>AEIPLKYGATNEGKRQDPAMQKFRDNRLGAFIHWGLYAIPGGEWNGKVYGGAAEWLKSWAKVPADEWLKLMDQWNPTKFDAKKWAKMAKEMGTKYVKITTKHHEGFCLWPSKYTKYTVANTPYKRDILGELVKAYNDEGIDVHFYFSVMDWSNPDYRYDIKSKEDSIAFSRFLEFTDNQLKELATRYPTVKDFWFDGTWDASVKKNGWWTAHAEQMLKELVPGVAINSRLRADDKGKRHFDSNGRLMGDYESGYERRLPDPVKDLKVTQWDWEACMTIPENQWGYHKDWSLSYVKTPIEVIDRIVHAVSMGGNMVVNFGPQADGDFRPEEKAMATAIGKWMNRYGKAVYACDYAGFEKQDWGYYTRGKNDEVYMVVFNQPYSERLIVKTPKGITVEKATLLTTGEDITVVETTRNEYNVSVPKKNPGEPYVIQLKVRAAKGTKSIYR[4x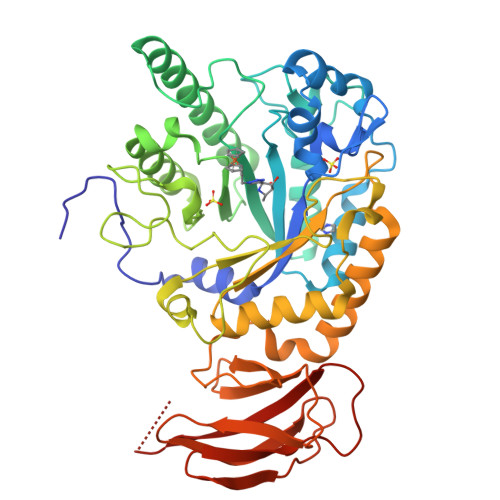]Here, crystal structures of human NLRP14 pyrin-domain variants are reported. Structurally, NLRPs share a conserved tripartite domain architecture consisting of an N-terminal pyrin domain, a central NACHT domain (with reference to its initial identification in NAIP, CIITA, Het-E and TP1) and a C-terminal leucine-rich repeat (LRR) domain. Pyrin domains belong to the death-domain superfamily, which includes the CARDs, the death-effector domains (DEDs) and the death domains (DDs) in addition to the PYDs. The death-domain fold consists of six antiparallel α-helices packed around a highly conserved hydrophobic core with Greek-key topology.

To investigate the functional role of the human NLRP14 PYD, we set out to crystallize the wild-type protein. The asymmetric unit is built up as a tetrameric arrangement resulting from a dimerization of dimers. Each of the four crystallographically independent NLRP14 PYD monomer structures adopts a canonical pyrin-domain fold with its N-terminal helices α1–α5. By contrast, the typical C-terminal α6 helix is not present as a separate secondary-structure element. Instead, the two C-terminal helices α5 and α6 combine to form an extended stem-helix, which we refer to as stem-helix α5/6. The dimer encompasses an extensive interface area of 890 Å2. We concluded from these experiments that wild-type NLRP14 PYD predominantly exists as a monomer in solution, with a monomer:dimer ratio of approximately 83:17% as judged from chromatogram peak areas. Nonetheless, the dimer constitutes only a minor fraction as shown by gel-filtration chromatography. Together with the thermal stability experiments, we conclude that the wild-type NLRP14 PYD will be mostly monomeric, with its C-terminal α6 helix contributing to the hydrophobic core only transiently.

>GSHMADSSSSSFFPDFGLLLYLEELNKEELNTFKLFLKETMEPEHGLTPWNEVKKARREDLANLMKKYYPGEKAWSVSLKIFGKMNLKDLCERAKEEINWSAQLE[4x]>NNNGACUUAAGUC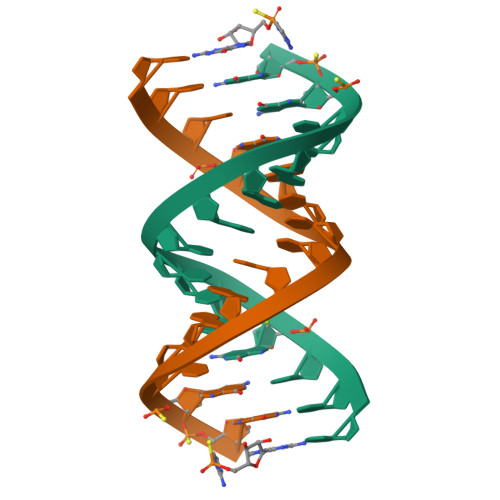GG[2x]> MNGVYDVGGTDGLGPINRPADEPVFRAEWEKVAFAMFPATFRAGFMGLDEFRFG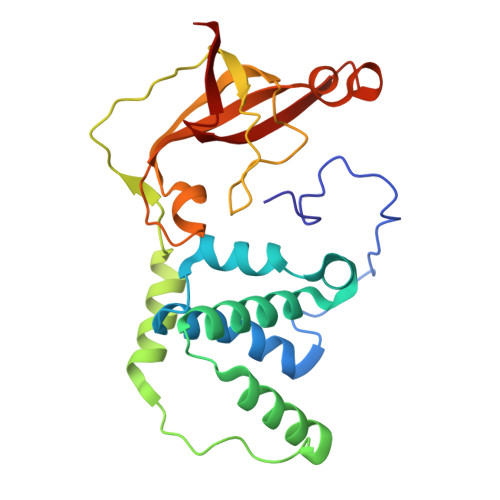IEQMNPAEYLESPYYWHWIRTYIHHGVRTGKIDLEELERRTQYYRENPDAPLPEHEQKPELIEFVNQAVYGGLPASREVDRPPKFKEGDVVRFSTASPKGHARRARYVRGKTGTVVKHHGAYIYPDTAGNGLGECPEHLYTVRFTAQELWGPEGDPNSSVYYDCWEPYIELVDT3'-deoxy-3'-(L-threonylamino)adenosine | C14 H21 N7 O5 | 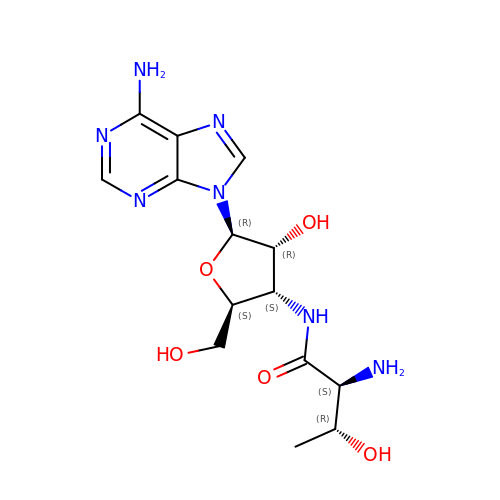JYCQZCJEBNTMCV-JHJLZTHQSA-N> MSKNEEMEGKMFIGGLSWDTTKKDLKDYFSKFGEVVDCTLKLDPITGRSRGFGFVLFKESESVDKVMDQKEHKLNGKVIDPKRAKAM;> MEGKMFIGGLSWDTTKKDLKDY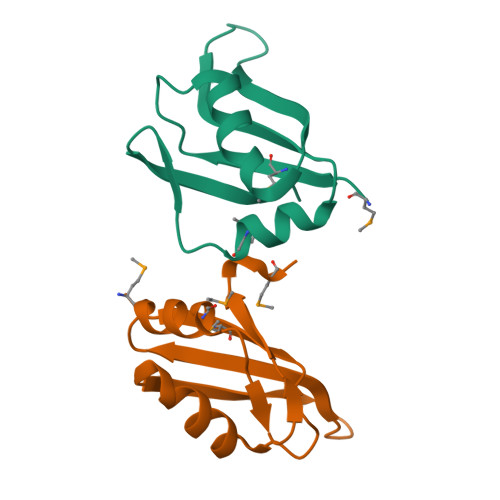FSKFGEVVDCTLKLDPITGRSRGFGFVLFKESESVDKVMDQKEHKLNGKVIDPKRAKAMA>[6x]MPKTDRVIEEITDYVLEKEITSAEAYTTAGHVLLDTLGCGILALRYPECTKLLGPIVPGTTVPNGSKVPGTSYVLDPVRAAFNIGC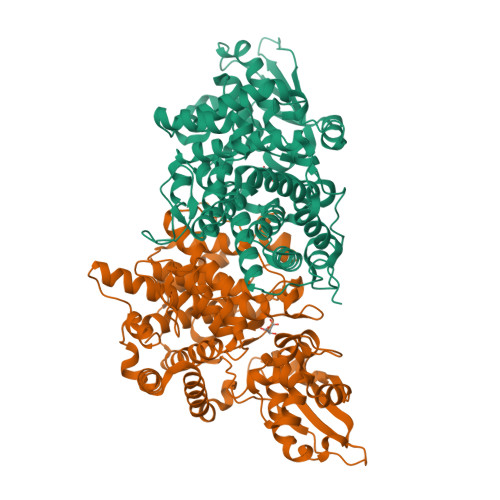MIRWLDYNDTWLAAEWGHPSDNLGGILAAADYVSRVRLSEGKEPLTVRDVLEMMIKAHEIQGVLALENSLNRVGLDHVLFVKVATTAVAAKLLGGGREEIKNALSNAWIDNAALRTYRHSPNTGSRKSWPAGDATSRGVHLALMSLKGEMGYPTALSAPGWGFQDVLFNKKEIKLARPLDAYVMENVLFKVSYPAEFHAQTAAESAVILHPQVKNRIDEIDRVVIRTHESAIRIIDKKGPLHNPADRDHCLQYITAIGLLFGDITAQHYEAETANDPRIDKLRDKMEVTENKTYTEDYLKPDKRSISNAVQVHFKDGTSTEMVECEFPLGHRFRREEAVPKLLEKFSDNLKTHFPDKQHKHIYERCTSYETLQTMRVNEFVDMFCM6-{[3-({[2-(3-fluorophenyl)ethyl]amino}methyl)phenoxy]methyl}-4-methylpyridin-2-amine 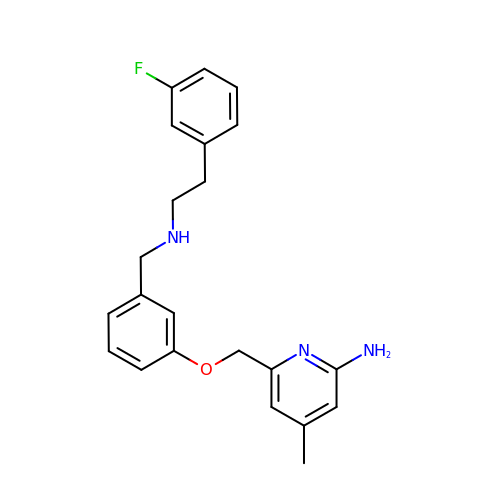| C22 H24 F N3 O | DDZKIKXHCIUETL-UHFFFAOYSA-N> MNQCPEHSQLTALG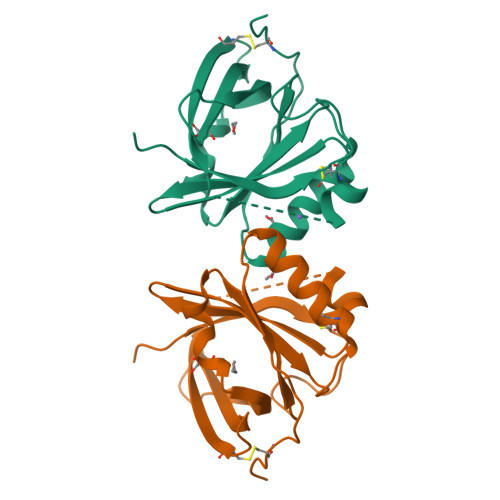MDDTETPEPHLGLWYFIAGAASTTEELATFDPVDNIVFNMAAGSAPRQLQLRATIRTKSGVCVPRKWTYRLTEGKGNMELRTEGRPDMKTDLFSSSCPGGIMLKETGQGYQRFLLYNRSPHPPEKCVEEFQSLTSCLDFKAFLVTPRNQEACPLSSK> EIFSQELTQREANVKKVHENLEELQKKLD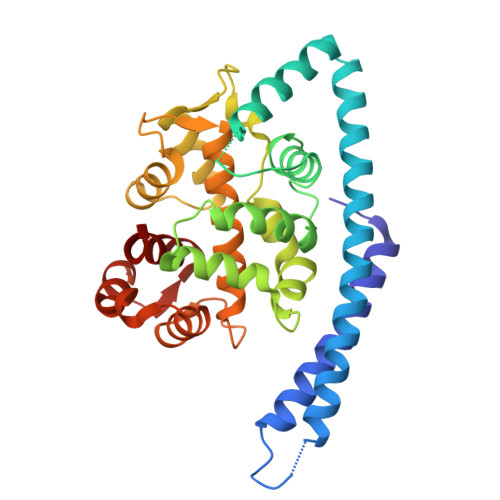HTSFAHKEDRDRLEAQIAQKEQEQKAKLAEYDQKVQNEFDARERAEREREAARGDAAAEKQRLASLLKDLEDDASGYNRLRPSKPMLSEEDTNILRQLFLSSAVSGSGKFSFQDLKQVLAKYADTIPEGPLKKLFVMVENDTKGRMSYITLVAVANDLAALVADFRKIDTNSNGTLSRKEFREHFVRLGFDKKSVQDALFRYADEDESDDVGFSEYVHLGLCLLVLRILYAFADFDKSGQLSKEEVQKVLEDAHIPESARKKFEHQFSVVDVDDSKSLSYQEFVMLVLLMFHDD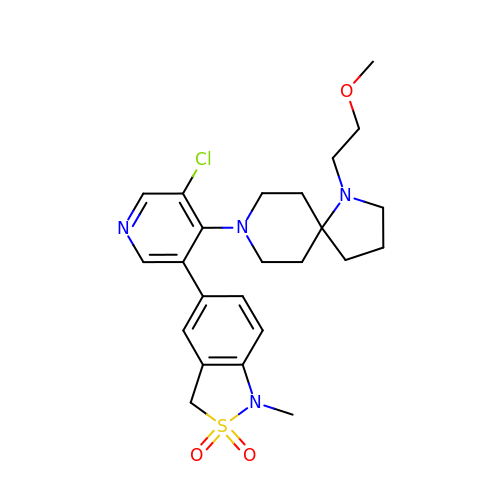5-[5-chloranyl-4-[1-(2-methoxyethyl)-1,8-diazaspiro[4.5]decan-8-yl]pyridin-3-yl]-1-methyl-3~{H}-2,1-benzothiazole 2,2-dioxide | C24 H31 Cl N4 O3 S | GRKOQLWARQVTPO-UHFFFAOYSA-N> MFEARLVQGSILKKVLEALKDLINEACWDIS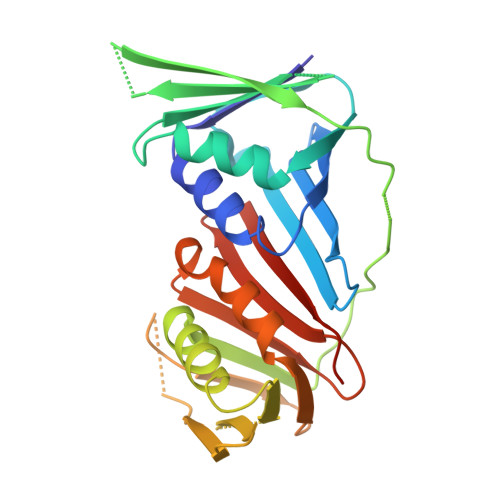SSGVNLQSMDSSHVSLVQLTLRSEGFDTYRCDRNLAMGVNLTSMSKILKCAGNEDIITLRAEDNADTLALVFEAPNQEKVSDYEMKLMDLDVEQLGIPEQEYSCVVKMPSGEFARICRDLSHIGDAVVISCAKDGVKFSASGELGNGNIKLSQTSNVDKEEEAVTIEMNEPVQLTFALRYLNFFTKATPLSSTVTLSMSADVPLVVEYKIADMGHLKYYLAPKIEDEE2-{2-[(4-carbamimidoylphenyl)carbamoyl]-6-methoxypyridin-3-yl}-5-{[(2S)-1-hydroxy-3,3-dimethylbutan-2-yl]carbamoyl}benzoic 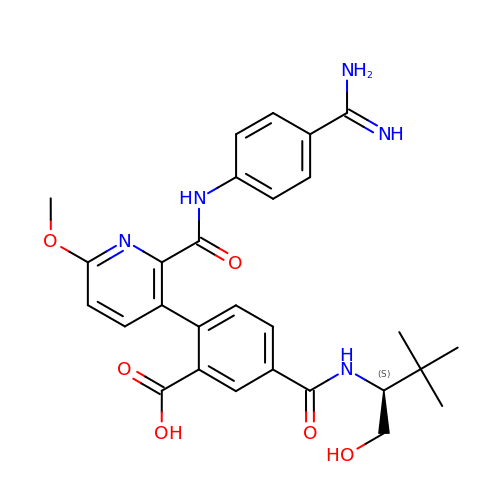acid | C28 H31 N5 O6 | KPACBFJTZSMBKD-OAQYLSRUSA-N> MALSGHVLIDPARLPRDTGPELMWAPSLRNSLRVSPEALELAEREAERARSERWDRCAQVLKNRLLRVELDGIMRDHLARAEEIRQDLDAVVAFSDGLESMQVRSPSTGGRSAPAPPSPSPAQPFTRLTGNAQYAVSISPTDPPLMVAGSLAQTLLGNLYGNINQWVPSFGPWYRTMSANAMQRRVFPKQLRGNLNFTNSVSLKLMTEVVAVLEGTTQDFFSDVRHLPDLQAALILSVAYLLLQGGSSHQQRPLPASREELLELGPESLEKIIADLKAKSPGGNFMILTSGNKEARQSIAPLNRQAAYPPGTFADNKIYNLFVGAGLLPTTAALNVPGAAGRDRDLVYRIANQIFGEDVPPFSSHQWNLRVGLAALEALMLVYTLCETANLAEAATRRLHLSSLLPQAMQRRKPAMASAGMPGAYPVQTLFRHGELFRFIWAHYVRPTVAADPQASISSLFPGLVLLALELKLMDGQAPSHYAINLTGQKFDTLFEIINQKLLFHDPAAMLAARTQLRLAFEDGVGVALGRPSPMLAAREILERQFSASDDY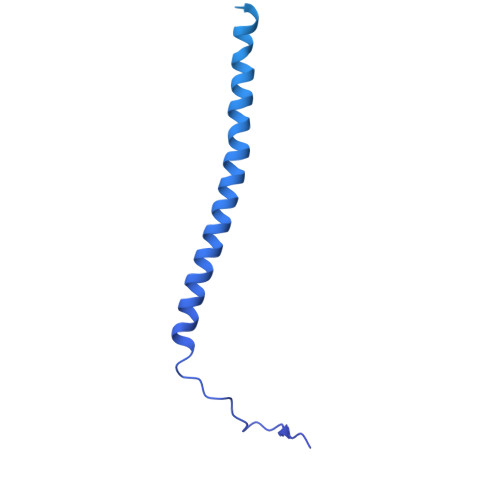DRLYFLTLGYLASPVAPS>[3x]AQVINTFDG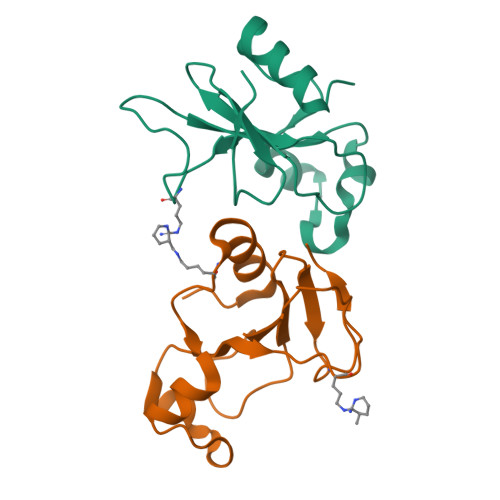VADYLQTYHKLPDNYITKSEAQALGWVASKGNLADVAPGKSIGGDIFSNREGKLPGKSGRTWREADINYTSGFRNSDRILYSSDWLIYKTTDHYQTFTKIR> GSVGPKTGE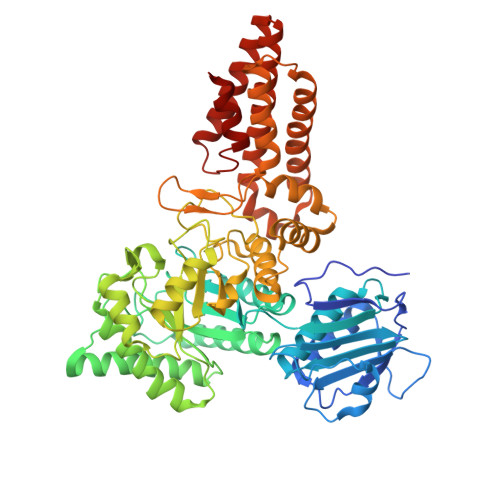ENQVLVPNLNPTPENLEVVGDGFKITSSINLVGEEEADENAVNALREFLTANNIEINSENDPNSTTLIIGEVDDDIPELDEALNGTTAENLKEEGYALVSNDGKIAIEGKDGDGTFYGVQTFKQLVKESNIPEVNITDYPTVSARGIVEGFYGTPWTHQDRLDQIKFYGENKLNTYIYAPKDDPYHREKWREPYPESEMQRMQELINASAENKVDFVFGISPGIDIRFDGDAGEEDFNHLITKAESLYDMGVRSFAIYWDNIQDKSAAKHAQVLNRFNEEFVKAKGDVKPLITVPTEYDTGAMVSNGQPRAYTRIFAETVDPSIEVMWTGPGVVTNEIPLSDAQLISGIYDRNMAVWWNYPVTDYFKGKLALGPMHGLDKGLNQYVDFFTVNPMEHAELSKISIHTAADYSWNMDNYDYDKAWNRAIDMLYGDLAEDMKVFANHSTRMDNKTWAKSGREDAPELRAKMDELWNKLSSKEDASALIEELYGEFARMEEACNNLKANLPEVALEECSRQLDELITLAQGDKASLDMIVAQLNEDTEAYESAKEIAQNKLNTALSSFAVISEKVAQSFIQEALS> PVDFTGYWKMLVNENFE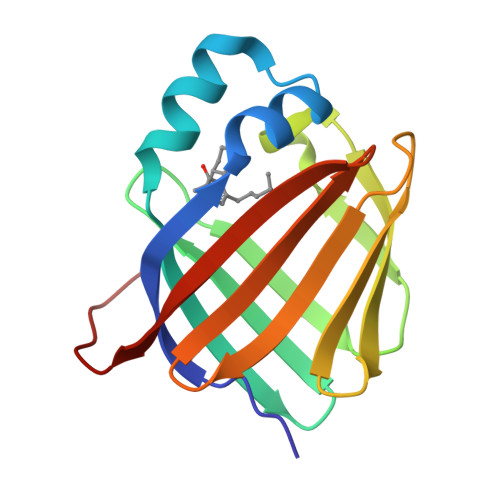EYLRALDVNVALRKIANLLKPDKEIVQDGDHMIIRTLSTFRNYIMDFQVGKEFEEDLTGIDDRKCMTTVSWDGDKLQCVQKGEKEGRGWTQWIEGDELHLEMRVEGVVCKQVFKKVQHHHHHH>[2x]GAMVKIIKKPKDVTALENATVAFEVSVSHDTVPVKWFHKSVEIKPSDKHRLVSERKVHKLMLQNISPSDAGEYTAVVGQLECKAKLFVETLHITKTMKNIEVPETKTASFECEVSHFNVPSMWLKNGVEIEMSEKFKIVVQGKLHQLIIMNTSTEDSAEYTFVCGNDQVSATLTVTPIMITSMLKDINAEEKDTITFEVTVNYEGISYKWLKNGVEIKSTDKCQMRTKKLTHSLNIRNVHFGDAADYTFVAGKATSTATLYVVEA

Evidence accumulated over the past two decades has identified titin as a main coordinator of cardiac muscle homeostasis, and its dysfunction through genetic mutation as an important factor in cardiomyopathy. For this, we examined the unique mSNP T2850I in the I-band domain of titin I10, as a paradigm of an alteration in a general component of the titin chain. Domain I10 does not support specific interactions or have any known specialized roles, so it does not constitute an a priori sensitive locus of the chain. In previous studies, we have shown that the T2580I mSNP destabilizes the affected immunoglobulin (Ig) domain in titin, I10, and speculated that this instability increases the vulnerability of titin to proteolysis in situ potentially leading to myocardial damage.

I19–I11 crystals were produced in (c) 0.1 M Tris HCl pH 8.5, 30% (w/v) PEG 4000, 0.2 M MgCl2; (d) 0.1 M Bis-Tris propane pH 8.5, 20% (w/v) PEG 3350, 0.2 M sodium acetate. A three-dimensional model from (c) was to 1.9 Å with Rfactor/Rfree = 19.28/22.83%; and from (d) to 1.53 Å with an Rfactor/Rfree = 16.15/19.65%. Three molecular copies were obtained in two space groups that agreed in showing I9–I11 in an extended conformation. In I9–I11, the component domains follow a regular arrangement, where domains display relative torsion angles of 45°–68° and are connected by short, two-residue sequences (TL and PI, respectively). In each Ig-pair, the domain interface is consistently formed by the A'B β-turn of the N-terminal domain slotting between the BC and FG loops of the C-terminal domain. Here, domains interact directly through a limited number of contacts (section S2). Both I9–I10 and I10–I11 interfaces consist of a central hydrophobic residue contributed by the linker sequence (TL; PI), flanked by two polar interactions between loop residues from the neighbouring domains (inset). In addition, electrostatic potential maps of single domains in the I9–I11 tandem revealed that the N- and C-terminal poles of all domains are, respectively, positively and negatively charged. This suggests that an electrostatic component further assists the organization of these Ig domains within the titin chain. Residue T2850 is buried within the I10–I11 interface (burial fraction of side chain is 0.79 as calculated with FoldX).>[2x]MAKAHIELTINGHPVEALVEPRTLLIHFIREQQNLTGAHIGCDTSHCGACTVDLDGMSVKSCTMFAVQANGASITTIEGMAAPDGTLSALQEGFRMMHGLQCGYCTPGMIMRSHRLLQENPSPTEAEIRFGIGGNLCRCTGYQNIVKAIQYAAAKINGVPFEEAAE;>MNIQTTVEPTSAERAEKLQGMGCKRKRVEDIRFTQGKGNYVDDVKLPGMLFGDFVRSSHAHARIKSIDTSKAKALPGVFAVLTAADLKPLNLHYMPTLAGDVQAVLADEKVLFQNQEVAFVVAKDRYVAADAIELVEVDYEPLPVLVDPFKAMEPDAPLLREDIKDKMTGAHGARKHHNHIFRWEIGDKEGTDATFAKAEVVSKDMFTYHRVHPSPLETCQCVASMDKIKGELTLWGTFQAPHVIRTVVSLISGLPEHKIHVIAPDIGGGFGNKVGAYSGYVCAVVASIVLGVPVKWVEDRMENLSTTSFARDYHMTTELAATKDGKILAMRCHVLADHGAFDACADPSKWPAGFMNICTGSYDMPVAHLAVDGVYTNKASGGVAYRCSFRVTEAVYAIERAIETLAQRLEMDSADLRIKNFIQPEQFPYMAPLGWEYDSGNYPLAMKKAMDTVGYHQLRAEQKAKQEAFKRGETREIMGIGISFFTEIVGAGPSKNCDILGVSMFDSAEIRIHPTGSVIARMGTKSQGQGHETTYAQIIATELGIPADDIMIEEGNTDTAPYGLGTYGSRSTPTAGAATAVAARKIKAKAQMIAAHMLEVHEGDLEWDVDRFRVKGLPEKFKTMKELAWASYNSPPPNLEPGLEAVNYYDPPNMTYPFGAYFCIMDIDVDTGVAKTRRFYALDDCGTRINPMIIEGQVHGGLTEAFAVAMGQEIRYDEQGNVLGASFMDFFLPTAVETPKWETDYTVTPSPHHPIGAKGVGESPHVGGVPCFSNAVNDAYAFL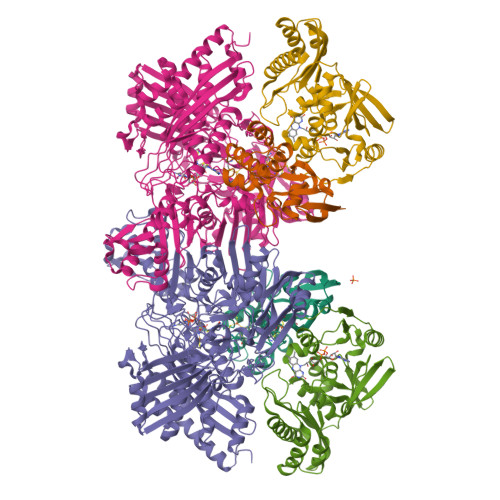NAGHIQMPHDAWRLWKVGEQLGLHV[2x];>[2x]MIPGSFDYHRPKSIADAVALLTKLGEDARPLAGGHSLIPIMKTRLATPEHLVDLRDIGDLVGIREEGTDVVIGAMTTQHALIGSDFLAAKLPIIRETSLLIADPQIRYMGTIGGNAANGDPGNDMPALMQCLGAAYELTGPEGARIVAARDYYQGAYFTAIEPGELLTAIRIPVPPTGHGYAYEKLKRKIGDYATAAAAVVLTMSGGKCVTASIGLTNVANTPLWAEEAGKVLVGTALDKPALDKAVALAEAITAPASDGRGPAEYRTKMAGVMLRRAVERAKARAKN>GSHMDIQVQVNIDDNGKNFDYTYTVTTESELQKVLNELMDYIKAAGAARVRISITARTSSEAEKFAAILRKVFAELGYND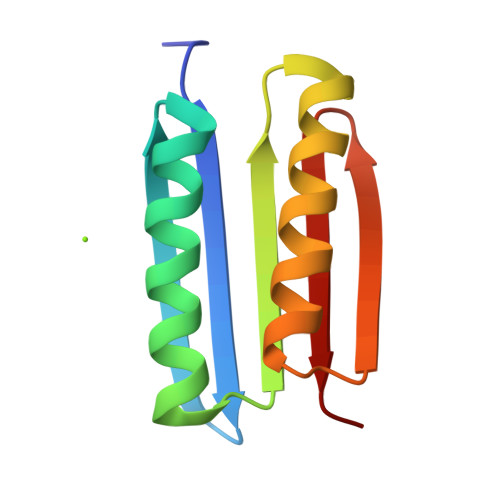INVTFDGDTVTVEGQLE[2x]Avapritinib | C26 H27 F N10 | 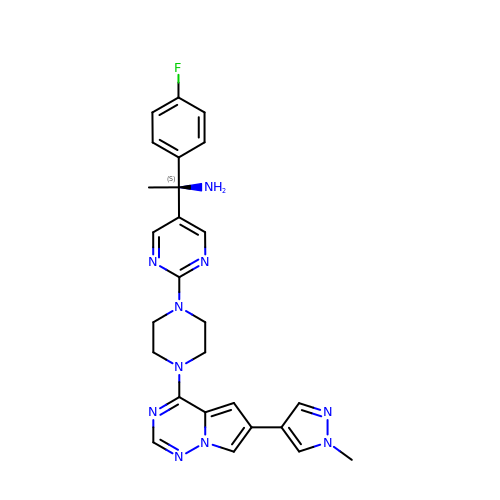DWYRIWUZIJHQKQ-SANMLTNESA-N> MKQSKVFIPTMRDVPSEAEAQSHRLLLK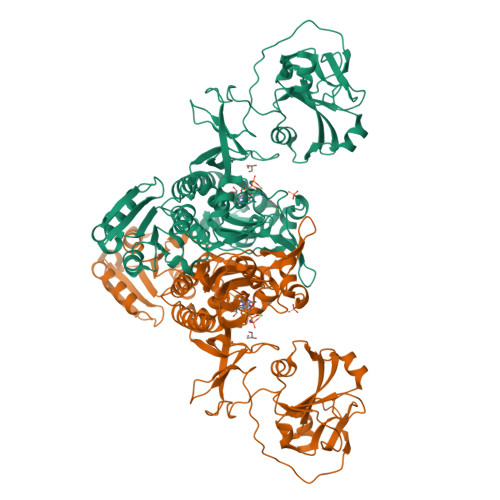SGLIKQSTSGIYSYLPLATRVLNNITAIVRQEMERIDSVEILMPALQQAELWEESGRWGAYGPELMRLQDRHGRQFALGPTHEELVTSIVRNELKSYKQLPMTLFQIQSKFRDEKRPRFGLLRGREFIMKDAYSFHADEASLDQTYQDMYQAYSRIFERVGINARPVVADSGAIGGSHTHEFMALSAIGEDTIVYSKESDYTANIEKAEVVYEPNHKHSTVQPLEKIETPNVKTAQELADFLGRPVDEIAKTMIFKVDGEYIMVLVRGHHEINDIKLKSYFGTDNIELATQDEIVNLVGANPGSLGPVIDKEIKIYADNFVQDLNNLVVGANEDGYHLINVNVGRDFNVDEYGDFRFILEGEKLSDGSGVAHFAEGIEVGQVFKLGTKYSESMNATFLDNQGKAQPLIMGCYGIGISRTLSAIVEQNHDDNGIVWPKSVTPFDLHLISINPKKDDQRELADALYAEFNTKFDVLYDDRQERAGVKFNDADLIGLPLRIVVGKRASEGIVEVKERLTGDSEEVHIDDLMTVITNKYDNLK> ST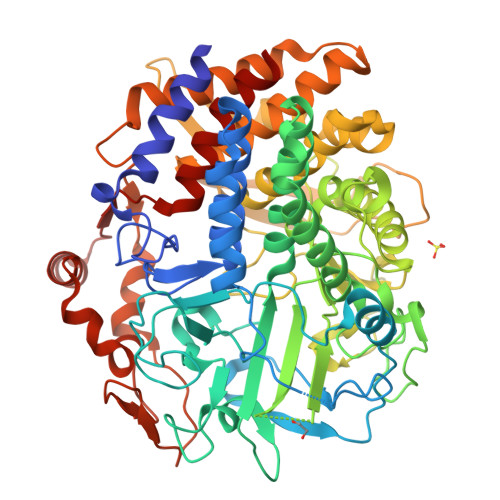PSVLGEYGQRFMWLWNKIHDPANGYFNQDGIPYHSVETLICEAPDYGHLTTSEAFSYYVWLEAVYGKLTGDWSKFKTAWDTLEKYMIPSAEDQPMRSYDPNKPATYAGEWETPDKYPSPLEFNVPVGKDPLHNELVSTYGSTLMYGMHWLMDVDNWYGYGKRGDGVSRASFINTFQRGPEESVWETVPHPSWEEFKWGGPNGFLDLFIKDQNYSKQWRYTDAPDADARAIQATYWAKVWAKEQGKFNEISSYVAKAAKMGDYLRYAMFDKYFKPLGCQDKNAAGGTGYDSAHYLLSWYYAWGGALDGAWSWKIGSSHVHFGYQNPMAAWALANDSDMKPKSPNGASDWAKSLKRQIEFYRWLQSAEGAIAGGATNSWNGRYEKYPAGTATFYGMAYEPNPVYHDPGSNTWFGFQAWSMQRVAEYYYVTGDKDAGALLEKWVSWVKSVVKLNSDGTFAIPSTLDWSGQPDTWNGAYTGNSNLHVKVVDYGTDLGITASLANALLYYSAGTKKYGVFDEGAKNLAKELLDRMWKLYRDEKGLSAPEKRADYKRFFEQEVYIPAGWIGKMPNGDVIKSGVKFIDIRSKYKQDPDWPKLEAAYKSGQAPEFRYHRFWAQCDIAIANATYEILFGNQ> GSHFEEGERVLAKHSDCFYEA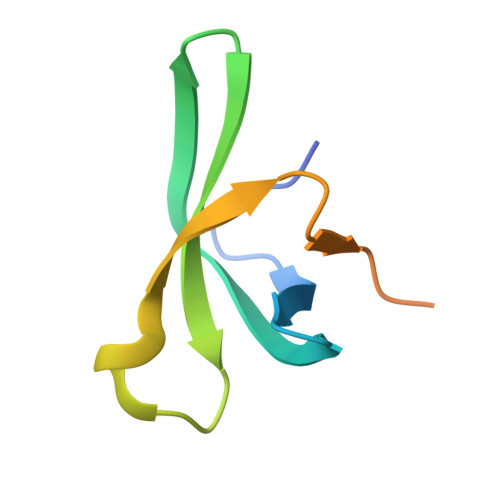KVLKVEFKDNEWKYFVHYIGWNKSWDEWIRLDCLLKHSDENIEKQKEQGLKQQG> MATSITTTQSTRQYPLSRYDDRNIADPILRAELRKEVMLMCESNDKNLTIYYVLPDEQYRPDLLAYRMWGIAELRWVVTLAAGLEDESQGMTVGKKLKLPPATWIREMIRH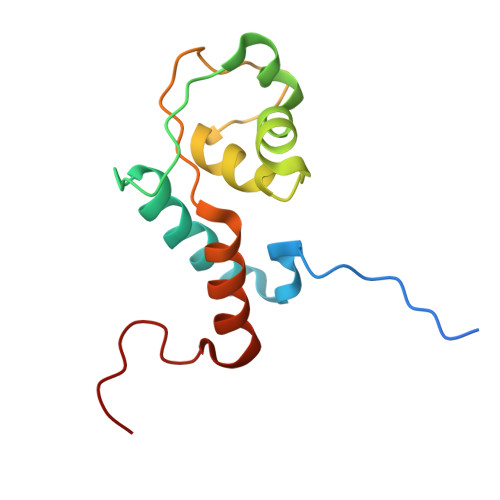FQYDGQVIGTLSIA> GPSGAADKAGTRENQPAVVHLQGQGSAIQVKNDLSGGVLNDWSRITMNPKVFKLHPRSGELEVLVDGTYFIYSQVEVYYINFTDFASYEVVVDEKPFLQCTRSI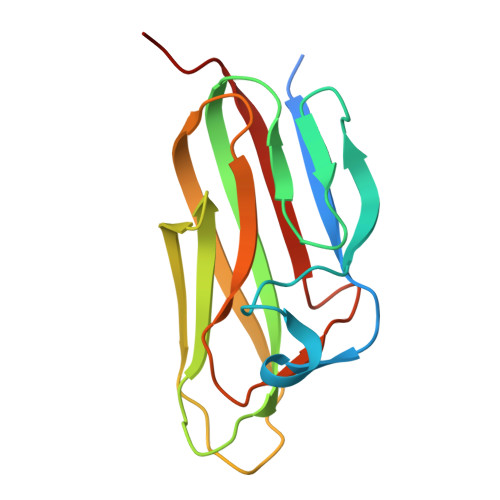ETGKTNYNTCYTAGVCLLKARQKIAVKMVHADISINMSKHTTFFGAIRLGEAPAS> RRTLWTTPDTSPNCKMSTEKDSKLTLTLTKCGSQVLGNVSLLAVTGEYHQMTATTKKDVKISLLFDENGILLPSSSLSKDYWNYRSDDSIVSQKYNNAVPFMPNLTAYPKPSAQNAKNYSRTKIISNVYLGALTYQPVIITIAFNQETENGCAYSITFT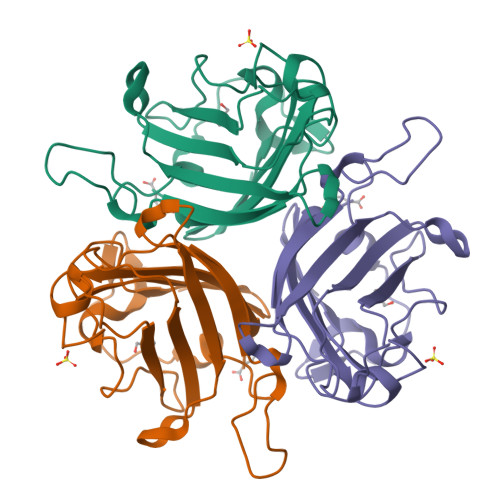FTWQKDYSAQQFDVTSFTFSYLTQ> L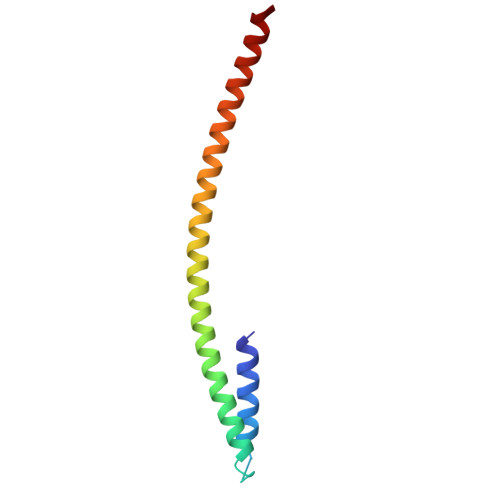LSALEDLEVLSRELIEMLAISRNQKLLQLEEENQVLELLIHRDGDFQELMKLALNQGKVHHEMQALEKEVEKRDSDIQQLQKQLKEAEQILATAVYQAK>AIAMTHPDISVDVLVIGAGPTGLGAAKRLNQIDGPSWMIVDSNETPGGLASTDVTPEGFLYDVGGHVIFSHYKYFDDCLDEALPKEDDWYTHQRISYVRCQGQWVPYPFANNISMLPKEEQVKCIDGMIDAALEARVANTKPKTFDEWIVRMMGTGIADLFMRPYNFKVWAVPTTKMQCAWLGERVAAPNLKAVTTNVILGKTAGNWGPNATFRFPARGGTGGIWIAVANTLPKEKTRFGEKGKVTKVNANNKTVTLQDGTTIGYKKLVSTMAVDFLAEAMNDQELVGLTKQLFYSSTHVIGVGVRGSRPERIGDKCWLYFPEDNCPFYRATIFSNYSPYNQPEASAALPTMQLADGSRPQSTEAKEGPYWSIMLEVSESSMKPVNQETILADCIQGLVNTEMLKPTDEIVSTYHRRFDHGYPTPTLEREGTLTQILPKLQD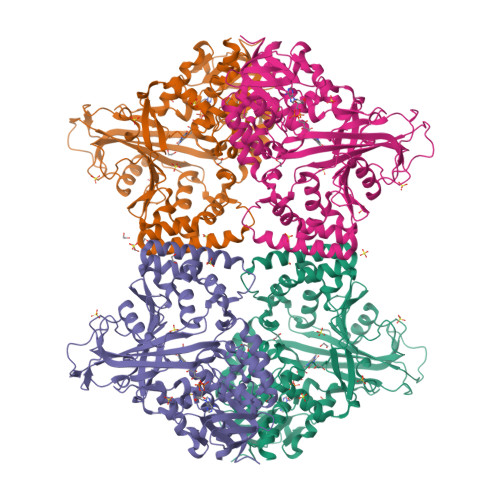KDIWSRGRFGSWRYEVGNQDHSFMLGVEAVDNIVNGAVELTLNYPDFVNGRQNTERRLVDGAQVFAKSKAQ[4x]> VEP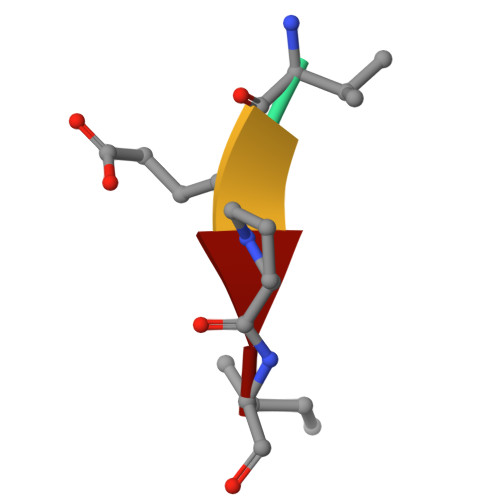I> GPHMASMLEAKFEEASLFKRIIKGFKDCVQLVNFQCKEDGIIAQAVDDSRVLLVSLEIGVEAFQEYRCDHPVTLGMDLTSLSKILRCGNNTDTLTLIADNTPDSIILLFEDTKKDRIAEYSLKLMDIDADFLKIEELQYDSTLSLPSSEFSKIVRDLSQLSDSINIMITKETIKF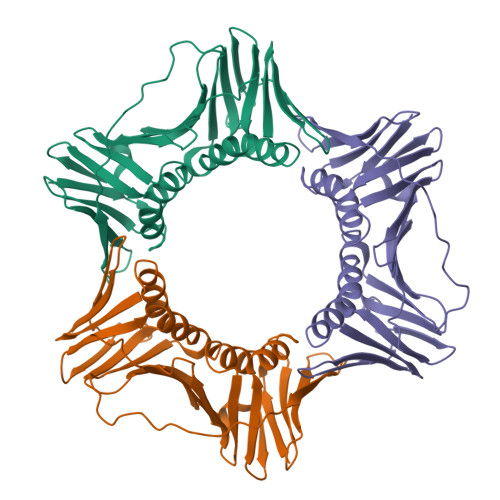VADGDIGSGSVIIKPFVDMEHPETSIKLEMDQPVDLTFGAKYLLDIIKGSSLSDRVGIRLSSEAPALFQFDLKSGFLQFFLAPKFNDEE> SMSDVTEQGAAEGGGRRARGEGRGAAARRASRTGGGPGPSLPYIQRRIREYEVLDEEGLQLIERNADVVLEEIGIEFRDDAEALDLWKAAGADVRGQRVHFPKGLCRELLKTAPKDFTWHARNPERNAQIGGKATVFAPVYGPPFVRDLDGNRRYATIEDFRNFVKLAYMAPSMHSSGGTVCEPVDIAVNKRHLDMVYSHIRYSDKPFMGSVTAPERAEDTVAMAKILFGDDFVENNAVTLNLINANSPMVFDETMLGAAKVYARHNQACVVSPFILSGAMSPVTVAGTL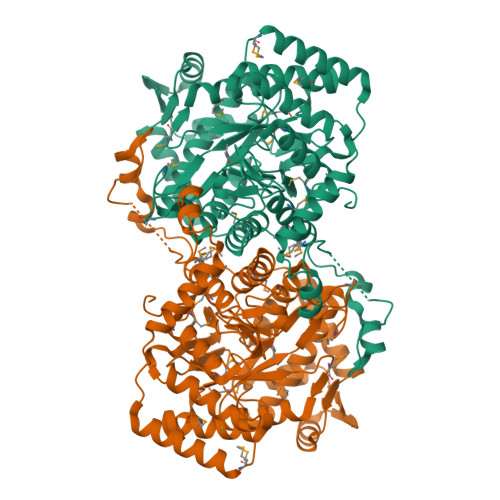TQILAEVLAGAAFTQLIRKGAPVLFGTFAASISMQSGAPTFGTPEPSLVSYGAAQLARRLGLPFRTGGSLCGSKVPDAQAAHESANTLNMTLLAGTNFVLHAAGWLEGGLVSSYEKFMIDQDQLGMMQKMAEGVDLSEDAQALDAIREVGPGSHYLGCAHTQANFQSAFYRSPLADNNSFEQWEIEGEKRIEQRANALARSWLEHYEAPYLDPAIDEALKEFIAKRKDSMPDAFT>AVGIFVIIFGIALFFLAMKVSGLVGTNLSDGYTMKAQFDNVNGLKPRAKVTMSGVTIGRVDSITLDPVTRLATVTFDLDGKLTSFNAEQLKEVQKNALDELRYSSDYTQATPAQQKTMEQQLISNMNSITSIDEDAYIMVATNGLLGEKYLKIVPGGGLNYLKRGDTISNTQGTMDLEDLISK[6x];>MNTIAWLGRLVIERIRGIGVAALMLLQIIFSLPSAGGFGRFVYQMHRVGVMSLLIITVSGLFIGLVLGLQGYSILVNVGSESMLGTMVSLTLLRELAPVVAALLFAGRAGSALTAEIGSMKQSEQLASMEMIGVDPLKQIVSPRLWAGIVSLPMLTVIFAAIGIVGGKLVGVDFLGVDEGSFWSGMQNNVQFGHDVVNGIIKSIVF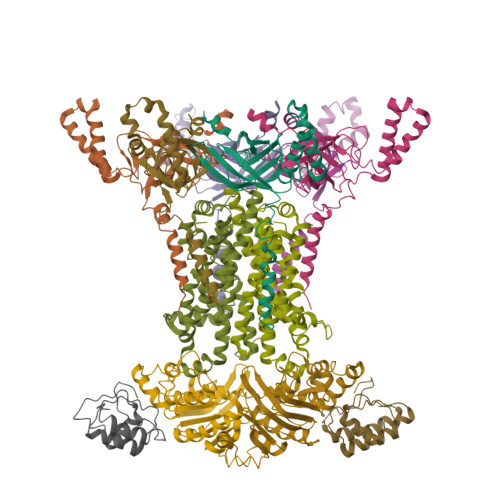ALLCTWIAVFQGYACDPTPEGIATAMTRTVVYSSLCVLGFDFVLTAVMFGG[2x];>[2x]LIEVKNLSFNRGERVIYDNISLNIRRGQITAIMGPSGTGKTTLLRLIGGQLVPDQGEVLLDGKDIAQMSRQRARMGMLFQSGALFTDMSVYENVAFPIRAHTLSENLIAELVALKLESVGLRGTEQLMPTELSGGMNRRVALARAIALDPDLIMYDEPFAGQDPIVKGVLTRLIRSLREALDLTTIIVSHDVPETLSIADYIYVVAEGKIQGEGTPEELQAYASPFVKQFLTG;>VQYLNQELVVSGKIDFENAEQQYQAGLAIIKKQTSFPLIVDLKQLEHGNTLALAVLVQWLRQTPQKSGLHFKNVPEKMLKIIQACHLQEDLHL[2x]> SDELYRQSLEIISRYLREQATGAKDTKPMGRSGATSRKALETLRRVGDGVQRNHETAFQGMLRKLDIKNEDDVKSLSRVMIHVFSDGVTNWGRIVTLISFGAFVAKHLKTINQESCIEPLAES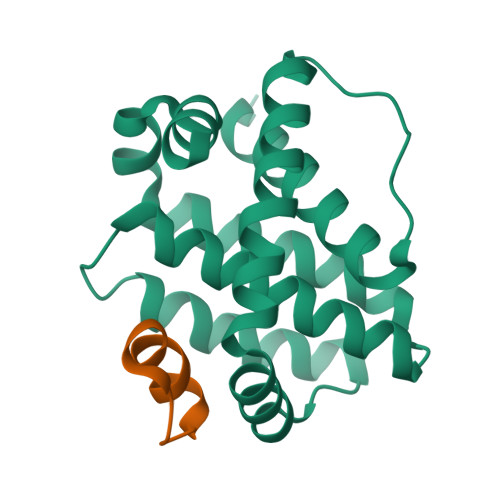ITDVLVRTKRDWLVKQRGWDGFVEFFHVE;> PPEIAWLADAVGLKDA2-[2-fluoranyl-4-[[2-fluoranyl-4-[2-(methylcarbamoyl)pyridin-4-yl]oxy-phenyl]carbamoylamino]phenyl]sulfanylethanoic 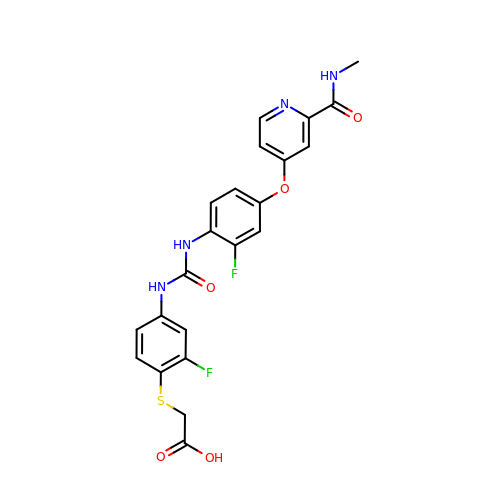acid | C22 H18 F2 N4 O5 S | LUCVAGIVDZCQRA-UHFFFAOYSA-N>[2x]MSTLETWPQVIINTYGTPPVELVSGKGATVTDDQGNVYIDLLAGIAVNALGHAHPAIIEAVTNQIGQLGHVSNLFASRPVVEVAEELIKRFSLDDATLAAQTRVFFCNSGAEANEAAFKIARLTG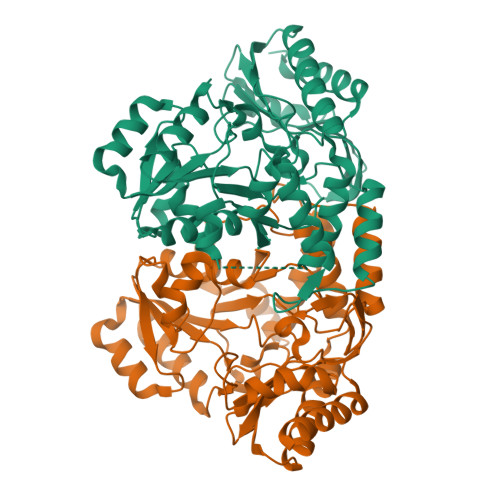RSRILAAVHGFHGRTMGSLALTGQPDKREAFLPMPSGVEFYPYGDTDYLRKMVETNPTDVAAIFLEPIQGETGVVPAPEGFLKAVRELCDEYGILMITDEVQTGVGRTGDFFAHQHDGVVPDVVTMAKGLGGGLPIGACLATGRAAELMTPGKHGTTFGGNPVACAAAKAVLSVVDDAFCAEVARKGELFKELLAKVDGVVDVRGRGLMLGVVLERDVAKQAVLDGFKHGVILNAPADNIIRLTPPLVITDEEIADAVKAIAETIALEHHHHHH> ETGMPLSC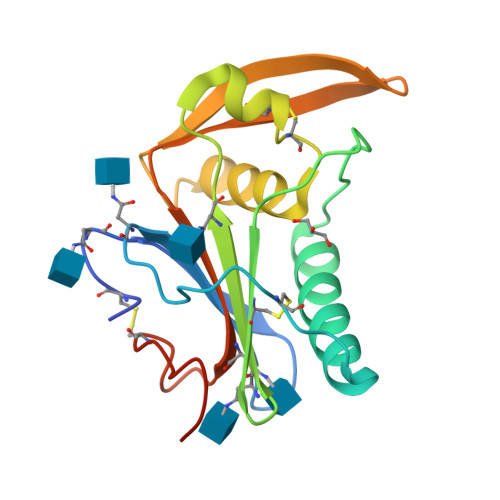SKNNSHHYIFVGNNSGLELTLTNTSLLNHKFCNLSDAHKRAQYDMALMSIVSTFHLSIPNFNQYEAMSCDFNGDNITVQYNLSHASAVDAANHCGTVANGILETFHKFFWSNNIKDAYQLPNQGKLAHCYSTSYQFLIIQNTTWEDHCTFSRPTGTKHHHHHH>[5x]MATFYEVIVRVPFDVE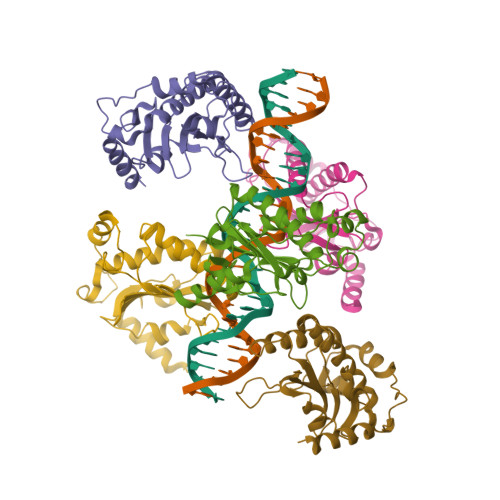EHLPGISDSFVDWVTGQIWELPPESDLNLTLVEQPQLTVADRIRRVFLYEWNKFSKQESKFFVQFEKGSEYFHLHTLVETSGISSMVLGRYVSQIRAQLVKVVFQGIEPQINDWVAITKVKKGGANKVVDSGYIPAYLLPKVQPELQWAWTNLDEYKLAALNLEERKRLVAQFLAESSQRS PHOSPHOMETHYLPHOSPHONIC ACID GUANOSYL ESTER | C11 H17 N5 O10 P2 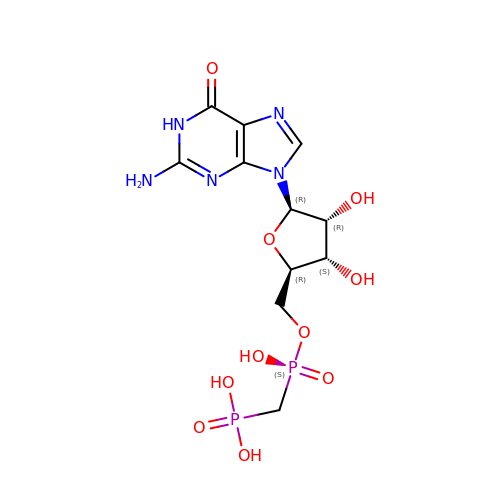| OCJWYBKRHNXUME-KQYNXXCUSA-N>[2x]QGLKDIYKDYFLIGVAVNQRNVSNAEQAALVKQEFNSITCENDMKPEPTEPQEGKFNWEAADRIANFCRTNGIKLRGHCLMWHSQIGRWMYSDNPTKEVFFQRMKNHIQAVVSRYKDVVYAWDVVNEAMTDDPKAEDPFRQSPLYKIAGDEFIAKAFQYAREADPNALLFYNDYNECDPVKSQRIYEMVKRMKENGVPIDGIGMQ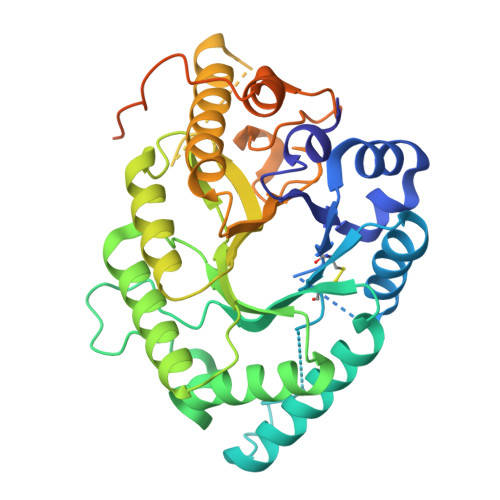GHYNIYGPTEAEIDAAITKYKSIVKHIHVTELDIRVNAEMGGQLQFSREGVAVSDSVKQHLADQYARVFNVLRKHRDVIDCVTFWNLSDRDSWLGQNNYPLPFDANYKPKMAYDYIKQMKAPAWPIPEKPKPNPNQQRQRRRGGFGGPQRPPFNPALAFAEQPGVKEDFVPSELNQPG>GPLGSMRTMVDSGQLTDPESARGKLLQTAAHLFRNKGFERTTVRDLASAVGIQSGSIFHHFKSKDEILRAVMEETIHYNTAMMRASLEEASTVRERVLALIRCELQSIMGGSGEAMAVLVYEWRSLSAEGQAHVLALRDVYEQIWLQVLGEAKAAGYIRGDVFITRRFLTGALSWTTTWF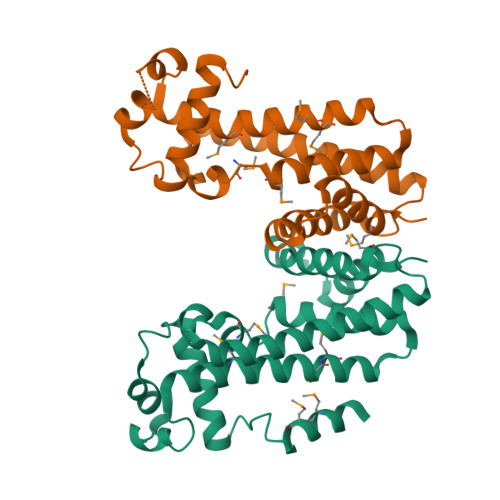RAQGSLTLEELAEEALLMVLKSD[2x]3-(1H-INDOL-3-YL)-6-(1H-PYRAZOL-4-YL)IMIDAZO[1,2-A]PYRAZINE | C17 H12 N6 | 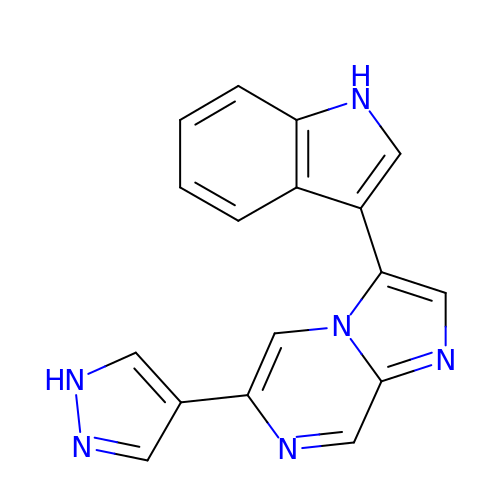ZCWUDZOATSSBCE-UHFFFAOYSA-N>[4x]GPLGSMTVKLDFEECLKDSPRFRASIELVEAEVSELETRLEKLLKLGTGLLESGRHYLAASRAFVVGICDLARLGPPEPMMAECLEKFTVSLNHKLDSHAELLDATQHTLQQQIQTLVKEGLRGFREARRDFWRGAESLEAALTHNAEVPRRRAQEAEEAGAALRTARAGYRGRA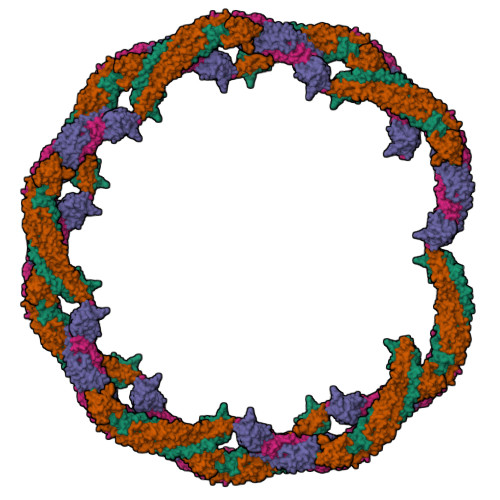LDYALQINVIEDKRKFDIMEFVLRLVEAQATHFQQGHEELSRLSQYRKELGAQLHQLVLNSAREKRDMEQRHVLLKQKELGGEEPEPSLREGPGGLVMEGHLFKRASNAFKTWSRRWFTIQSNQLVYQKKYKDPVTVVVDDLRLCTVKLCPDSERRFCFEVVSTSKSCLLQADSERLLQLWVSAVQSSIASAFSQARLDDSPRGPGQ N-[2-(3-methoxyphenyl)ethanimidoyl]-2-piperidin-4-yloxy-pyridine-3-carboxamide | C20 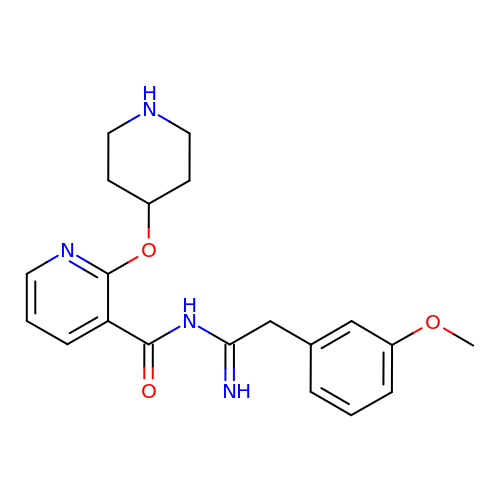H24 N4 O3 | GRWVIKXCGQEZMV-UHFFFAOYSA-N(2S)-2-AMINO-1-(5-TERT-BUTYL-1,3,4-OXADIAZOL-2-YL)PROPAN-1-ONE | 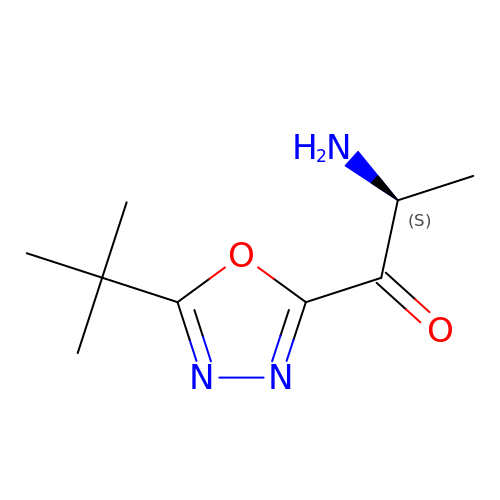C9 H15 N3 O2 | PVDZDTVFUVTTDU-YFKPBYRVSA-N>[2x]SMAALAPLPPLPAQFKSIQHHLRTAQEHDKRDPVV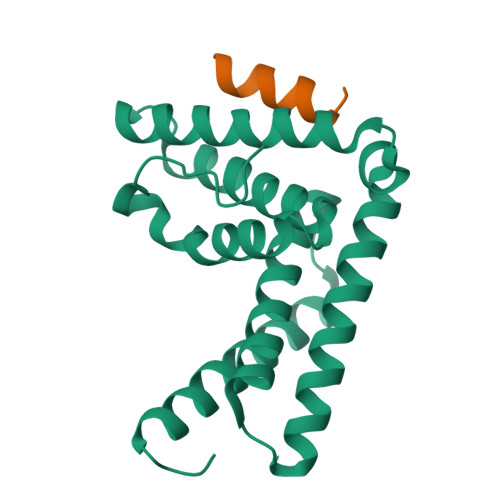AYYCRLYAMQTGMKIDSKTPECRKFLSKLMDQLEALKKQLGDNEAITQEIVGCAHLENYALKMFLYADNEDRAGRFHKNMIKSFYTASLLIDVITVFGELTDENVKHRKYARWKATYIHNCLKNGETP;>SVGTSVASAEQDELSQRLARLRDQV[2x]> MKKFIFATIFALASCAAQPAM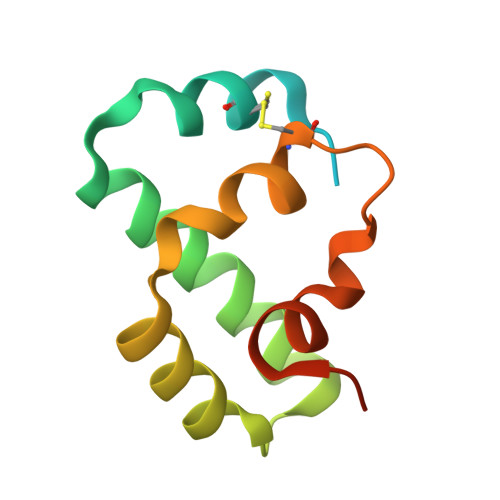AGYDKDLCEWSMTADQTEVETQIEADIMNIVKRDRPEMKAEVQKQLKSGGVMQYNYVLYCDKNFNNKNIIAEVVGELEHHHHHH>[4x]KKIFKPEELRQALMPTLEALYRQDPESLPFRQPVDPQLLGIPDYFDIVKNPMDLSTIKRKLDTGQYQEPWQYVDDVWLMFNNAWLYNRKTSRVYKFCSKLAEVFEQEIDPVMQSLG

Many proteins, including the EP300/CBP histone acetyltransferases (HATs), contain several targetable domains. EP300 and CBP broadly regulate the activity of other proteins through their protein acetyltransferase catalytic activity. These proteins contain several highly homologous domains, including KIX, bromodomains (BRDs) and HAT domains, through which they interact with, dock to, and acetylate target proteins, respectively. EP300/CBP are critical gene-regulatory targets in cancer, with existing high potency inhibitors of either the catalytic HAT domain or protein-binding bromodomain (BRD). Using crystallography, we identify the binding mechanism of the EP300/CBP-specific BRD inhibitor CCS1477 in complex with the EP300, CBP and BRD4 BRDs, and define components of the CCS1477 catalytic binding core that are required for compound activity.

To understand the structural basis for the observed differential binding affinities of CCS1477 between EP300/CBP and BRD4, we next solved the co-crystal structures of the respective bromodomains with CCS1477. As expected, CCS1477 binds through canonical hydrogen-bonding interactions of its dimethyl isoxazole moiety with a conserved asparagine residue in the acetyl-lysine (Kac) binding site (CBPN1168, EP300N1132, BRD4N140). A major difference, however, between the inhibitor binding pattern in EP300/CBP and BRD4 is the involvement of an arginine side chain (EP300R1137, CBPR1173) that interacts with the difluorophenyl ring of CCS1477 through Pi-cation interactions, while establishing an additional hydrogen-bond with the piperidinone oxygen. In EP300/CBP, an analogous tryptophan residue is not present, and instead the equivalent LPF shelf is less bulky and facilitates interaction with CCS1477. Superposition of CCS1477 as bound in the respective Kac sites reveals an altered binding pose, reflecting the reduced shape complementarity between CCS1477 and BRD4, as compared with EP300/CBP. CCS1477 produced a greater thermal shift with EP300 or CBP, as compared with BRD4. Further analysis of the binding energies by isothermal titration calorimetry (ITC) confirmed significantly stronger interaction of CCS1477 with the bromodomains of CBP and EP300 (Kd = 4.0 and 26 nM, respectively) than with BD1 of BRD4 (Kd = 403 nM). Thus, CCS1477 displays preferential binding to the bromodomains of EP300 and CBP, compared with BRD4. Since recombinant CBP BRD was more robust in biochemical assays and crystallization studies, Kd values were determined for all compound-CBP interactions by MST, and co-crystal structures of the CBP BRD with five of the seven analogues were determined. Thus, the difluorophenyl group is a critical moiety in the CCS1477 pharmacophore that facilitates potent interaction with the bromodomain of EP300/CBP and is required for efficacy in cell line models of G3MB.>[3x]MRGSHHHHHHGSMRFAIVVTGPAYGTQQASSAFQFAQALIADGHELSSVFFYREGVYNANQLTSPASDEFDLVRAWQQLNAQHGVALNICVAAALRRGVVDETEAGRLGLASSNLQQGFTLSGLGALAEASLTCDRVVQF;>[3x]MKRIAFVFSTAPHGTAAGREGLDALLATSALTDDLAVFFIADGVFQLLP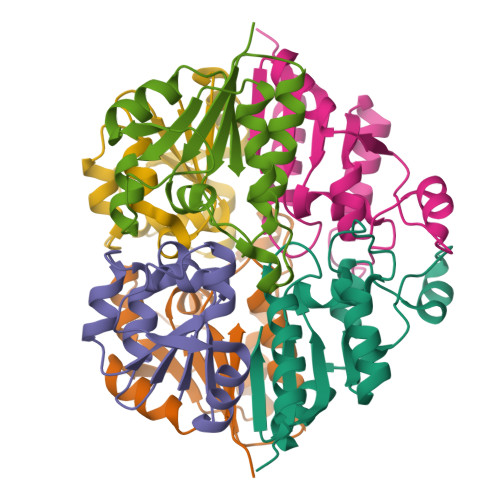GQKPDAVLARDYIATFKLLGLYDIEQCWVCAASLRERGLDPQTPFVVEATPLEADALRRELANYDVILRF;>[3x]MLHTLHRSPWLTDFAALLRLLSEGDELLLLQDGVTAAVDGNRYLESLRNAPIKVYALNEDLIARGLTGQISNDIILIDYTDFVRLTVKHPSQMAW> MGASAGLIRRGGGVFPDAVSLTLTPSRRVYGGSGRGDLLYENPDARRHSGRALGVLNGVRHSSQATMPESGQLYYRKLILHSRPPNGSCAGLQRHCHDTCNWSYLIPSLHR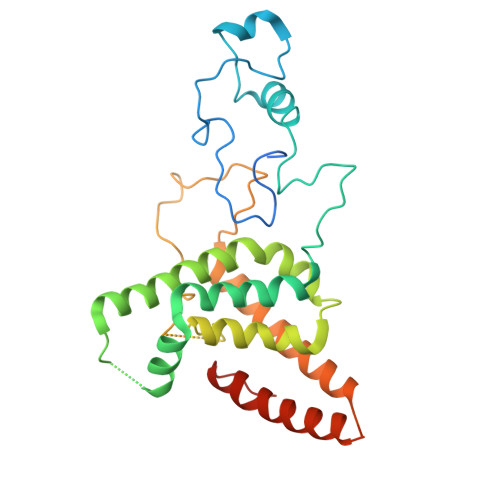CAESAISAKLWEKMCQLGLEDRSKAWVNLTQYERQRVRDGQNLYRYEVHQRLPLLEESIGWAQLDDLLGWFRSARRAWVRLPTSVTLSRESSEAGVASVVSPSSAMSCRLEGHADSRDTTPGRNQVFDTPERVEQLTEATVHRIREELQRLNRSERSDCEGSAAMRASARRLARDEELSRCVEEELGWHGVALQHRIPVPK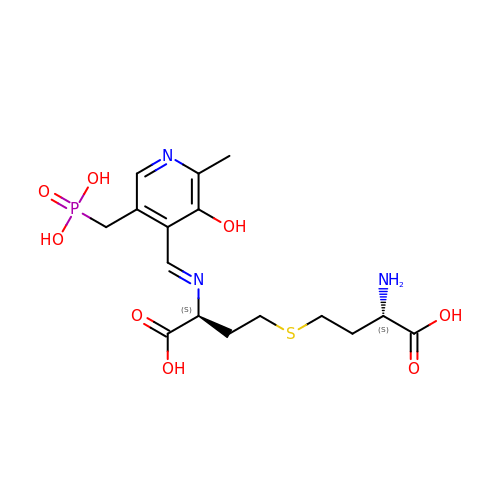(2~{S})-2-azanyl-4-[(3~{S})-3-[(~{E})-[2-methyl-3-oxidanyl-5-(phosphonomethyl)pyridin-4-yl]methylideneamino]-4-oxidanyl-4-oxidanylidene-butyl]sulfanyl-butanoic acid | C16 H24 N3 O8 P S | QGHPUHOZHNBFHZ-VNBISDOUSA-N>[4x]MPKTGREKRKSPENRFLRKLLKPDIERERLKAVNSIISIVFGTRRIAWAHLDRKLTVLDWQQSDRWSLMRGIYSSSVYLEEISSIISKMPKADFYVLEKTGLSIQNSSLFPILLHFHIMEAMLYALLNKTFAQDGQHQVLSMNRNAVGKHFELMIGDSRTSGKELVKQFLFDSILKADPRVFFPSDKIVHYRQMFLSTELQRVEELYDSLLQAIAFYELAVFDSQPLEHHHHHH;>[2x]MGHHHHHHGEFKALTRRLQVEPRLLSKQMAGCLEDCTRQAPESPWEEQLARLLQEAPGKLSLDVEQAPSGQHSQAQLSGQQQRLLAFFKCCLLTDQLPLAHHLLVVHHGQRQKRKLLTLDMYNAVMLGWARQGAFKELVYVLFMVKDAGLTPDLLSYAAALQCMGRQDQDAGTIERCLEQMSQEGLKLQALFTAVLLSEEDRATVLKAVHKVKPTFSLPPQLPPPVNTSKLLRDVYAKDGRVSYPKLHLPLKTLQCLFEKQLHMELASRVCV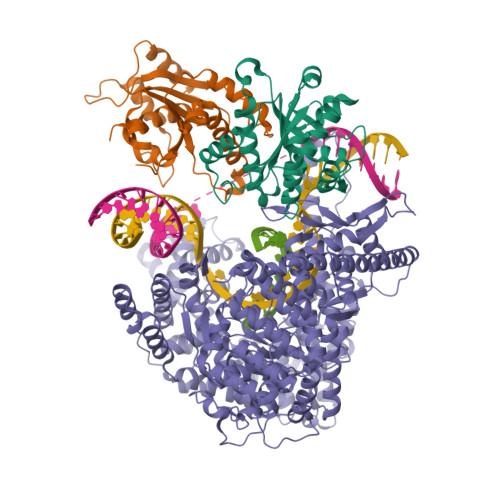VSVEKPTLPSKEVKHARKTLKTLRDQWEKALCRALRETKNRLEREVYEGRFSLYPFLCLLDEREVVRMLLQVLQALPAQGESFTTLARELSARTFSRHVVQRQRVSGQVQALQNHYRKYLCLLASDAEVPEPCLPRQYWEALGAPEALREQPWPLPVQMELGKLLAEMLVQATQMPCSLDKPHRSSRLVPVLYHVYSFRNVQQIGILKPHPAYVQLLEKAAEPTLTFEAVDVPMLCPPLPWTSPHSGAFLLSPTKLMRTVEGATQHQELLETCPPTALHGALDALTQLGNCAWRVNGRVLDLVLQLFQAKGCPQLGVPAPPSEAPQPPEAHLPHSAAPARKAELRRELAHCQKVAREMHSLRAEALYRLSLAQHLRDRVFWLPHNMDFRGRTYPCPPHFNHLGSDVARALLEFAQGRPLGPHGLDWLKIHLVNLTGLKKREPLRKRLAFAEEVMDDILDSADQPLTGRKWWMGAEEPWQTLACCMEVANAVRASDPAAYVSHLPVHQDGSCNGLQHYAALGRDSVGAASVNLEPSDVPQDVYSGVAAQVEVFRRQDAQRGMRVAQVLEGFITRKVVKQTVMTVVYGVTRYGGRLQIEKRLRELSDFPQEFVWEASHYLVRQVFKSLQEMFSGTRAIQHWLTESARLISHMGSVVEWVTPLGVPVIQPYRLDSKVKQIGGGIQSITYTHNGDISRKPNTRKQKNGFPPNFIHSLDSSHMMLTALHCYRKGLTFVSVHDCYWTHAADVSVMNQVCREQFVRLHSEPILQDLSRFLVKRFCSEPQKILEASQLKETLQAVPKPGAFDLEQVKRSTYFFS> PSALDAIVA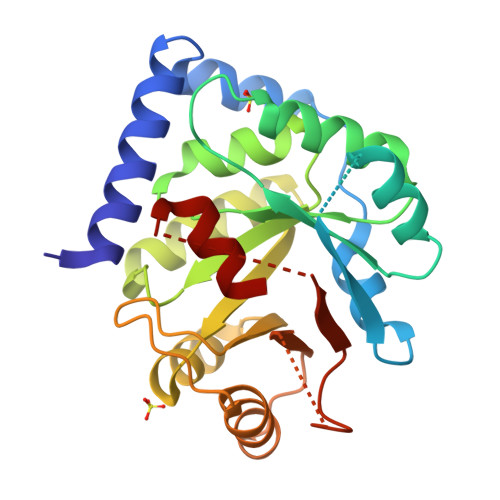DVREDVAAREAVVPFDEIKERAARAPPPRDVLAALRAPGVGIIAVYLRKSPSGLDVERDPIEYAKTAEKYAVALVVITDEKYHNGSYEDLEKIRSAVDIPVICFDFIVDPYQIYLARAYQADAIVLILSVLDDEQYRQLAAVAHSLNMGVIVDVHTEEELERALKAGAEIIGIVNQDLKTFEVDRNTAERLGRLARERGFTGVLLAIGGYSTKEELKSMRGLFDAVVIGESLMRAPDPEKAIRELVG>VGPKTGEENQVLVPNLNPTPENLEVVGDGFKITSSINLVGEEEADENAVNALREFLTANNIEINSENDPNSTTLIIGEVDDDIPELDEALNGTTAENLKEEGYALVSNDGKIAIEGKDGDGTFYGVQTFKQLVKESNIPEVNITDYPTVSARGIVEGFYGTPWTHQDR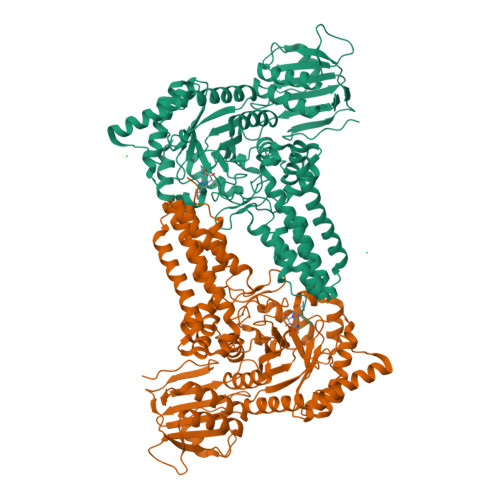LDQIKFYGENKLNTYIYAPKDDPYHREKWREPYPESEMQRMQELINASAENKVDFVFGISPGIDIRFDGDAGEEDFNHLITKAESLYDMGVRSFAIYWDDIQDKSAAKHAQVLNRFNEEFVKAKGDVKPLITVPTEYDTGAMVSNGQPRAYTRIFAETVDPSIEVMWTGPGVVTNEIPLSDAQLISGIYDRNMAVWWNYPVTDYFKGKLALGPMHGLDKGLNQYVDFFTVNPMEHAELSKISIHTAADYSWNMDNYDYDKAWNRAIDMLYGDLAEDMKVFANHSTRMDNKTWAKSGREDAPELRAKMDELWNKLSSKEDASALIEELYGEFARMEEACNNLKANLPEVALEECSRQLDELITLAQGDKASLDMIVAQLNEDTEAYESAKEIAQNKLNTALSSFAVISEKVAQSFIQEALSFDLTLI[2x]> GAMDPRVTMNEFEYLKLLGKGTFGKVILVKEKATGRYYAMKILKKEVIVAKDEVAHTLTENRVLQNSRHPFLTALKYSFQTHDRLC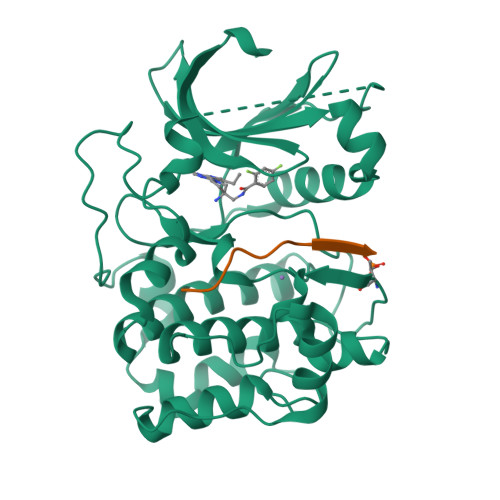FVMEYANGGELFFHLSRERVFSEDRARFYGAEIVSALDYLHSEKNVVYRDLKLENLMLDKDGHIKITDFGLCKEGIKDGATMKTFCGTPEYLAPEVLEDNDYGRAVDWWGLGVVMYEMMCGRLPFYNQDHEKLFELILMEEIRFPRTLGPEAKSLLSGLLKKDPKQRLGGGSEDAKEIMQHRFFAGIVWQHVYEKKLSPPFKPQVTSETDTRYFDEEFTAQMITITPPDQDDSMECVDSERRPHFPQFDYSASSTA;> GRPRTTSFAE> MLALGIEGTAHTLGIGIVSEDKVLANVFDTLTTEKGGIHPKEAAEHHARLMKPLLRKALSEAGVSLDDIDVIAFSQGPGLGPALRVVATAARALAVKYRKPIVGVNHCIAHVEITKMFGVKDPVGLYVSGGNTQVLALEGGRYRVFGETLDIGIGNAIDVFARELGLGFPGGPKVEKLAEKGEKYIELPYAVKGMDLSFSGLLTEAIRKYRSGKYRVEDLAYSFQETAFAALVEVTERAVAHTEKDEVVLVGGVAANNRLREMLRIMTEDRGIK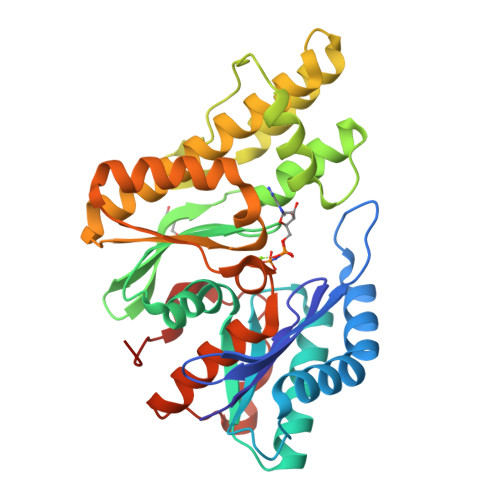FFVPPYDLCRDNGAMIAYTGLRMYKAGISFRLEETIVKQKFRTDEVEIVWHHHHHH>[2x]GIPKCPEDWGASSRTSLCFKLYAKGKHEKKTWFESRDFCRALGGDLASINNKEEQQTI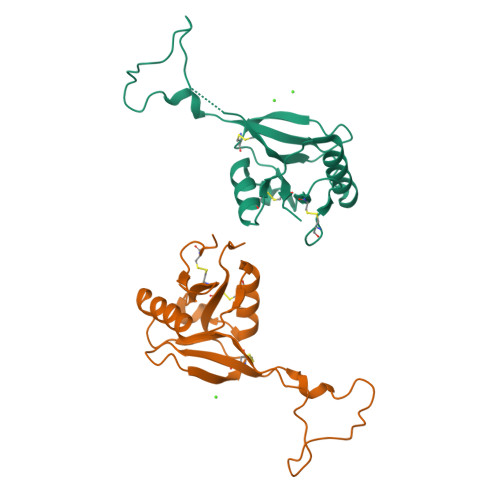WRLITASGSYHKLFWLGLTYGSPSEGFTWSDGSPVSYENWAYGEPNNYQNVEYCGELKGDPTMSWNDINCEHLNNWICQIQKGQTPKPD> SRN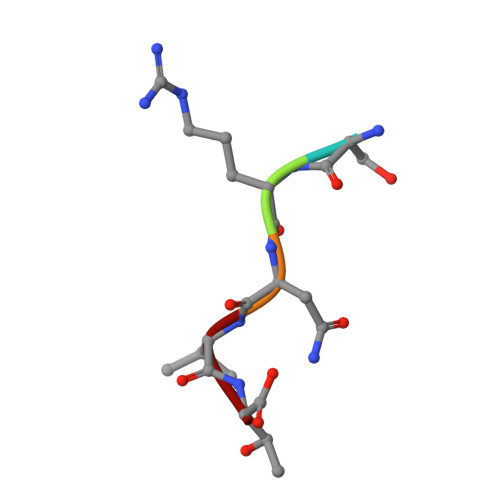VT> MTDQGLEGS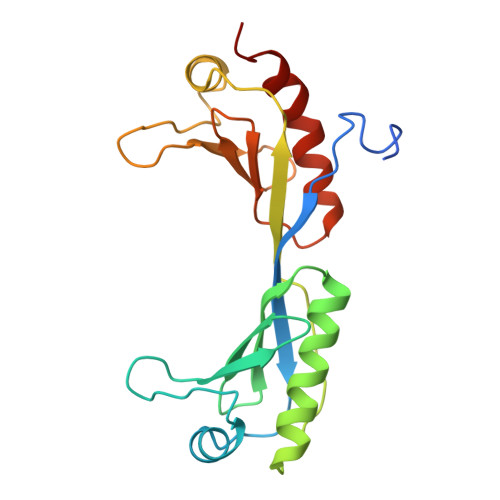NPVDLSKHPSGIVPTLQNIVSTVNLDCKLDLKAIALQARNAEYNPKRFAAVIMRIREPKTTALIFASGKMVCTGAKSEDFSKMAARKYARIVQKLGFPAKFKDFKIQNIVGSCDVKFPIRLEGLAYSHAAFSSYEPELFPGLIYRMKVPKIVLLIFVSGKIVITGAKMRDETYKAFENIYPVLSEFRKIQQ> MDYILGRYVKIARYGSGGLVGGGGKEQYVENLVLWENIIKTAYCFITPSSYTAALETANIPEKDFSNCFRFLKENFFIIPSEYNNSTENNRYSRNFLHYQSYGANPVLVQDKLKNAKVVILGCGGIGNHVSVILATSGIGEIILIDNDQIENTNLTRQVLF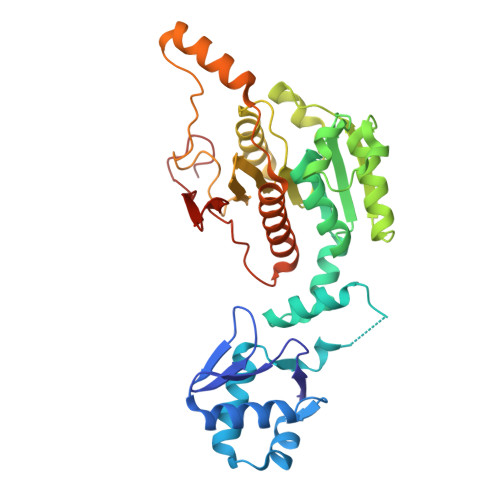SEDDVGKNKTEVIKRELLKRNSEISVSEIALNINDYTDLHKVPEADIWVVSADHPFNLINWVNKYCVRANQPYINAGYVNDIAVFGPLYVPGKTGCYECQKVVADLYGAEKENIDHKIKLINSRFKPATFAPVNNVAAALCAADVIKFIGKYSEPLSLNKRIGIWSDEIKIHSQNMGRSPVCSVCGN> GPGSEFRNKRATRGTYSPSAQEYCNPRLEMDNVLKPPPEER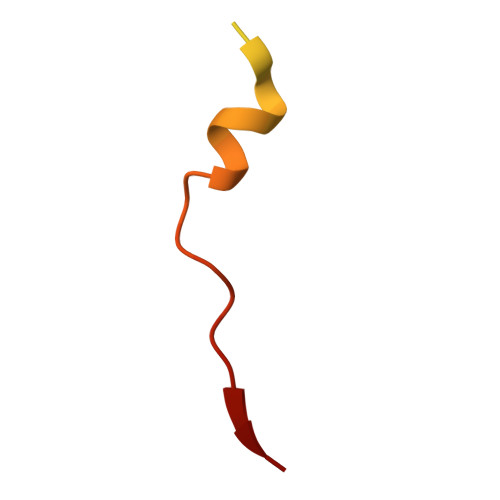LI> EEPPTVALTVPAAALLPDGALGESIVRGRRYLSDTPAQLPDFVGNGLACRHCHPGRDGEVGTEANAAPFVGVVGRFPQYSARHGRLITLEQRIGDCFERSLNGRALALDHPALIDMLAYMSWLSQGVPVGAVVAGHGIPTLTLEREPDGVHGEALYQARCLACHGADGSGTLDADGRYLFPPLWGPRSFNTGAGMNRQATAAGFIKHKMPLGADDSLSDEEAWDVAGFVLTHPRPLFQEPTGDASWSHPQFEK

Thiosulfate dehydrogenase (TsdA) catalyzes the oxidation of two thiosulfate molecules to form tetrathionate and is predicted to use an unusual cysteine-ligated heme as the catalytic cofactor. TsdA comprises two cytochrome c-like domains connected by a long unstructured linker. Each cytochrome domain contains one covalently bound heme molecule. The structural environment of the two hemes suggests a model for electron transfer in TsdA in which the electrons derived from thiosulfate oxidation are initially accepted by the heme in the N-terminal “catalytic” domain before being passed to the heme in the C-terminal “electron transfer” domain and then to an external electron acceptor protein positioned on the surface of TsdA near the exposed heme edge.

However, for TsdA co-crystallized with tetrathionate, the electron density in the active site could be confidently fitted, and this is the TsdA structure presented here. The presented structure was determined to 1.3 Å resolution from crystals grown at pH 4.6. In this structure, Cys123 is present as a cysteine S-sulfane conjugate rather than the cysteine S-thiosulfonate adduct expected from reaction with tetrathionate. The heme iron of the N-terminal domain heme is coordinated by the sulfane atom of the Cys123-S-sulfane conjugate and by His80. The ligands to the heme in the C-terminal domain are Met236 and His191. The packing of the two domains positions the two hemes close together, resulting in a nearest heme macrocycle edge-to-edge distance of 8.1 Å. The active site of TsdA co-crystallized with tetrathionate contains density that is well interpreted as a molecule of thiosulfate at 46% occupancy. The presence of thiosulfate in the crystallization environment is expected because it is formed as a product of the initial thiosulfonation of Cys123 by tetrathionate (Reaction 6). The thiosulfate molecule has bonding interactions with the amino acid side chains of Arg109, Arg119, and Ser127 as well as with the main chain amide group of Gly221 from the electron transfer domain. The thiosulfate molecule in the crystal structure plausibly occupies the position of the thiosulfate molecule in the first half-reaction because only a small movement of the thiosulfate would be needed to achieve the geometry expected in the disulfide bond-forming transition state: the attacking sulfur atom (thiosulfate sulfane atom) in line with the bond between the target sulfur atom (heme-ligating sulfur atom) and the leaving group (the heme iron).>MTQTYNADAIEVLTGLEPVRRRPGMYTDTTRPNHLGQEVIDNSVDEALAGHAKRVDVILHADQSLEVIDDGRGMPVDIHPEEGVPAVELILCISVVNALSKRVEVNVRRDGQVYNIAFENGEKVQDLQVVGTCGKRNTGTSVHFWPDETFFDSPRFSVSRLT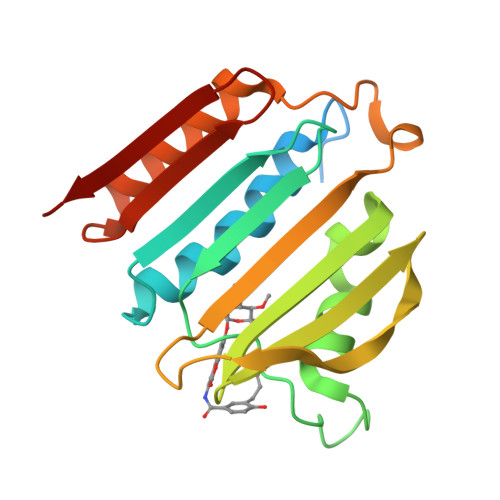HVLKAKAVLCPGVEITFKDEINNTEQRWCYQD[2x]6-[ethyl-[3-(2-methoxyethoxy)-4-propan-2-yl-phenyl]amino]pyridine-3-carboxylic acid | C20 H26 N2 O4 | 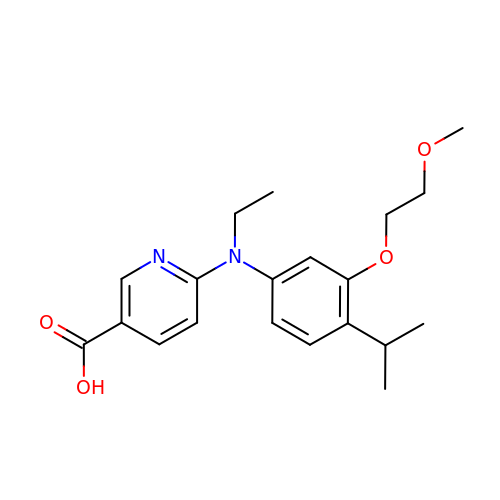VVNCNFPVMMKHFN-UHFFFAOYSA-N TrmK catalyzes the transfer of a methyl group from SAM to tRNA, producing m1A22-tRNA and SAH. SaTrmK is typical of class-I methyltransferases, with an N-terminal domain where the cofactor binds and methyl transfer takes place and a C-terminal domain likely involved in tRNA recognition. TrmK is essential for Staphylococcus aureus survival during infection but has no homolog in mammals, making it a promising target for antibiotic development. To shed light on the structural basis for cofactor binding and help inform future structure-based inhibitor design, crystals of SaTrmK apoenzyme, and the binary complexes SaTrmK:SAM and SaTrmK:SAH were obtained, and data were collected to a resolution of 1.3, 1.4, and 1.5 Å, respectively.

The electron density data for the SaTrmK apoenzyme showed clearly defined density near the active site that could not be fitted with any of the small molecules involved in purification or crystallization of the enzyme, suggesting it was carried through with SaTrmK from protein expression. Intriguingly, citrate could be fitted perfectly into the electron density, making polar contacts with the side chains of His27, Tyr29, and Asn59. It is possible the negatively charged groups of citrate are mimicking the phosphate group(s) of tRNA. DSF analysis indicated that citrate leads to an overall modest decrease in SaTrmK Tm that only becomes noticeable at high citrate concentrations, which is incompatible with the presumed tight binding required for the interaction to continue from protein expression to crystallization. Therefore, the significance of this observation, if any, is still elusive. In the absence of tRNA, SaTrmK contributes no background luminescence, as expected since the enzyme is not purified bound to SAH. This is evidenced by the crystal structure of the apoenzyme and no SAH detected by LC-MS after denaturation of SaTrmK which would have released any bound SAH. Superposition of the three structures revealed negligible effect of cofactor binding on Cα root-mean-square deviations (RMSDs), whose values were 0.15, 0.18, and 0.08 Å between SaTrmK and SaTrmK:SAM, SaTrmK and SaTrmK:SAH, and SaTrmK:SAM and SaTrmK:SAH, respectively. A superposition of the active sites of SaTrmK, SaTrmK:SAM, and SaTrmK:SAH shows there is local motion of some residues in order to accommodate the cofactor.

> GMISLNNRLTTVSRFLKQGTIADIGSDHAYLPIYAIQNHLCECGIAGEVIQGPFQAAVKNVAANQLVDRIDVRLGDGLSVIQPEDVIDNITICGMGGPLIAKILKDGQDKLSQHPRLILQSNIQTENLRQTLQQLNYEIIDEIIMEEKGHIYEIVVAEYSTELIELSSDELKFGPKLLNNKNEYFIKKWQRELEALYHIKSKLNTEQHHQRLAQINDEIAVIERVL> GQPQQVVVGVSGNGYVTRQQDGARITQRGVTHWTNPKSIVSIYFYLHQPTTADLSLYAKGHSEIKVSYGKKGFKVNLQSNDFTKVPVGSIDIRQAGYVRIDLQGVSKSGEGFGEIKQLIADNVTGKSNYVKDFSDYWGRRGPSVHLGYALPEGDTEWFYNEITVPKEGETMHSYYMAAGFGEGYFGMQYNSPTERRILFSVWSPFDTQNPKEIPDDQKIKLLRQGKDVHIGEFGNEGSGGQSYLKYPWKAGNTYKFLMQIRPDGNGNTTYTAYFYATDEKEWKLIASFLRPKTNTWYKRPHSFLENFSPEQGYLSREVFFGNQWARSKEGKWSRLTDATFTHDATASAQVRLDYQGGNTKDNRFYLKMGGFFNESVPM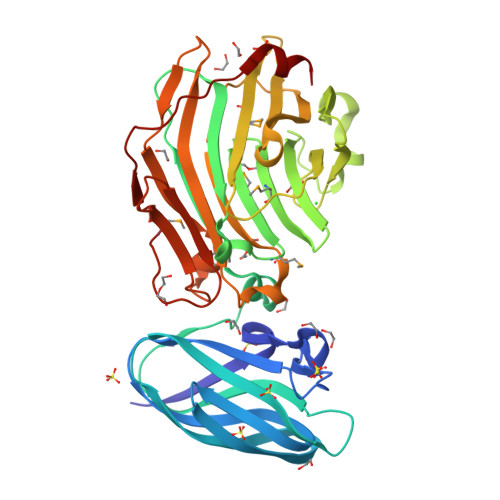GTKFYCKPTGKEPEIDWEALKQL>AMELIRIAMKKDLENDNSLMNKWATVAGLKNPNPLYDFLNHDGKTFNEFSSIVNIVKSQYPDREYELMKDYCLNLDVKTKAARSALEYADANMFFEIEDALIDSMISCSNMKSKEYGKVYKIHRELSKGEIDVFEASANIGKQRIKTAEMNIFSKMLLMYDCLNKGNFAPMMLLFQQIDLSEIKENRYLKNSFETRINVLLSNIYLNENNLELCREYAQKAISSTDTQRFLVFSYLTIGTSYIFSDFNLSKQNYLIGLKFAKGNPGFEEFFKRNLSFLNNFWNKENEWINYDSDAVTDMQEVIFELINHKELSKALQLLNKLEERDQNENELGFHYYLKGLITNEKEAFFKSVEYFKASQDKLSIKMPLIQLEKM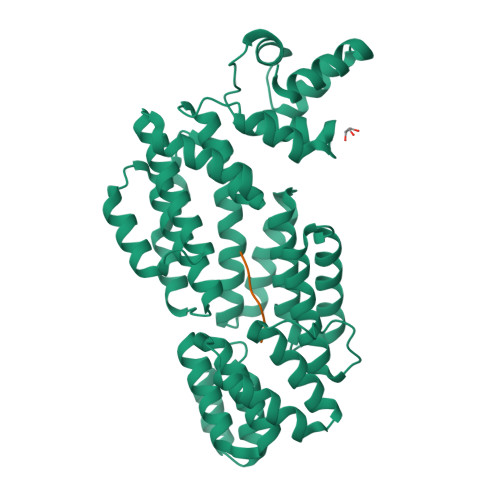GENPRLLKIITM[2x];>[2x]GIVRGA> MNTYLIDPRKNNDNSGERFTVDAVDITAAAKSAAQQILGEEFEGLVYRETGES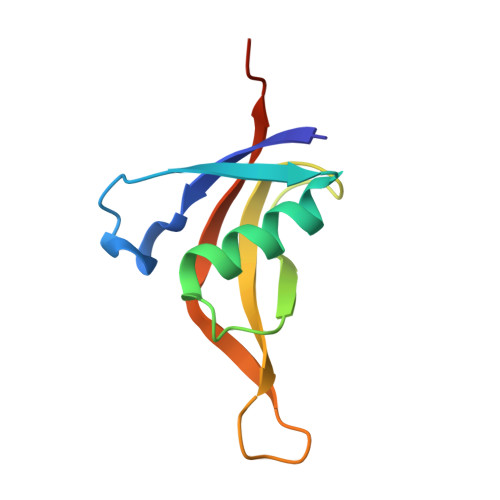NGSGMFQAYHHLHGTNRTETTVGYPFHVMELLEHHHHHH ChtII is a GH18 chitinase and possesses the greatest number of catalytic domains and chitin-binding domains in this family. Here we report the catalytic properties and the crystal structures of the catalytic domains of OfChtII, the ChtII derived from the Asian corn borer O. furnacalis. Analyzing the domain structure of the predicted protein with the SMART tool revealed that OfChtII contains five GH18 domains and seven CBM14-type chitin-binding modules (CBMs). The other two GH18 domains (C1 and C2) are predicted to be catalytically active (CAD).

To gain detailed insights into the substrate binding mode, catalysis defective mutants were constructed and crystallized. The inactive mutant, OfChtII-C2 E2180L, enabled us to obtain the enzyme–substrate complex structure at a resolution of 2.4 Å by soaking the crystal with chitooligosaccharide substrate (GlcNAc)5. The complex structure was similar to that of the wildtype enzyme, with an r.m.s. deviation of 0.17 Å based on the superimposition of 383 corresponding Cα atoms. The 2Fo − Fc map showed clear electron density for (GlcNAc)5 along the substrate-binding cleft from subsites −2 to +3. A close-up view of the enzymatic cleavage region showed that the sugar residue bound at subsite −1 adopted an unfavorable “boat” 1,4B conformation, which raises the free energy of the substrate. The aromatic residues Trp2067, Trp2138, and Trp2256 interacted hydrophobically with the −2, +1, and +2 sugar residues, respectively. Additionally, all of the acetamido groups pointed away from their corresponding sugar rings, which suggests an energetically favorable conformation. In particular, the C2-acetamido group of the −1 sugar pointed toward the catalytic residue Asp2178, and the O1 and O6 atoms of the −1 sugar formed hydrogen bonds with the side chains of Tyr2250 and Tyr2303/Asp2251, respectively. The O6 atom of the −2 sugar formed hydrogen bonds with the main-chain amides of both Trp2138 and Asp2139. In the substrate complex of the OfChtII-C2 mutant, the corresponding aspartate turned to the other side as a result of the mutation of catalytic glutamate, which abolished the hydrogen bond.

>ERFKVVCYYTNWAWYRPDNGKYTPGDINPELCTHIIYAFAVLDKEELVIKSHDIWLDVENKFYEKVTALKSHGVKVLLGLGGWDDSAGDKYSRLVNNVSARRKFVVHAVDFLEQYGFDGLDLDWLYPKCWQVECEKGPDSDKQGFADLVKELRKAFNRRGMLLSAAVSASKRVIDYAYNVPALSMNLDWISLMTYDYHGQWDKKTGHVAPMYVHDKDTDNTFNVNFTVNYWINKGADRKKLVVGVPFYGQSFSVVEGAGTGLGAPTYAGGEAGDETRARGFLSFYEICERVKVKGWKVHRDPGGRIGPYATHDDQWVSFDDDFMARHKAEYVRAMELGGSMAWSLDLDDFTGKYCGCGKAPLLTTINHVLRGKEAPPPCILHE[2x]> MNNLKPFIYYDWEKTILKNTKENYSINEIIPKTFFMELHGTKITNSTLNGTWKSWNLTNEGEGSYPVLKCIIDDGYLDMNFGASSEKIPLKNVWIKLCMKINPNSDGTYSIPEKSSSFYIKDNSLKISKDNLILDKYLNKLMLSYFKNNIKNIEMFINKSRIQTKVVGDLSLLGWNTENSVSFRTMNEFIKKDNLYPKDFKAVYSYRKMTFTATGTFDSWEMTTGADGRNIRFKCPIKYAVYDLDGDVFNSSTENFLLIQVDLTYFDSKTTINDPTGENDGKQFNLKIKTNDDKLKNVLIVTYNLTDTDGSMSSEDKDFLSLAFRNWFNENIQQFEQIFAYILLDETAKIPEYQWLKPTQISYGSASVETANDEPDLDASIFSAMSMVENNTNSTPSHAVDNRMLQLTKTQAAFGISFPLFIEHFLKQALLSSQFISVDDIVADINTLTITNNKQIIFGKVENSDGKNVDSSLKPGKLKLSLQNNLIVLELFDLTWEQGRGVTGHFDFRQEYELALESKSGKQIPILKVHDEPEIEYYVEEAQWKTNEDMIVSAVVGTVFSMILGASMKLAGSALSKAGKLIRSKATTIKGRKKIYINRSNVRQLRKDSGATEIELERINRRNSSIAAEDARLISNNGTTSIQTLGDMKKKPMSTGQRIAIGAKKIAGTAVMFGAVGLGMNFGEMLINYINAMENNDYSAIPGINSFMQQ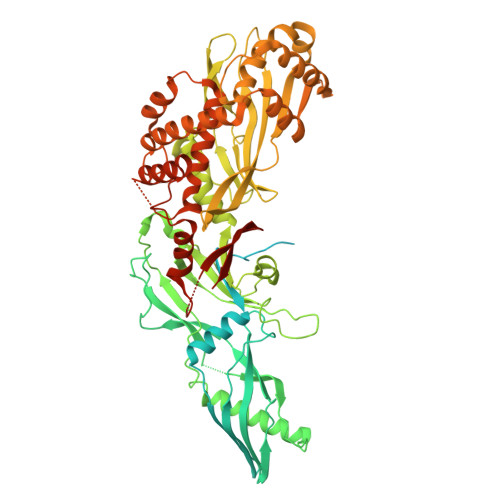CIGAMQWPDKDSELKVTFGKLQGIYLLGGTLEKNNKTDNK>[2x]ADILPANYVVKDRWKVLKKIGGGGFGEIYEAMDLLTRENVALKVESAQQPKQVLKMEVAVLKKLQGKDHVCRFIGCGRNEKFNYVVMQLQGRNLADLRRSQPRGTFTLSTTLRLGKQILESIEAIHSVGFLHRDIKPSNFAMGRLPSTYRKCYMLDFGLARQYTNTTGDVRPPRNVAGFRGTVRYASVNAHKNREMGRHDDLWSLFYMLV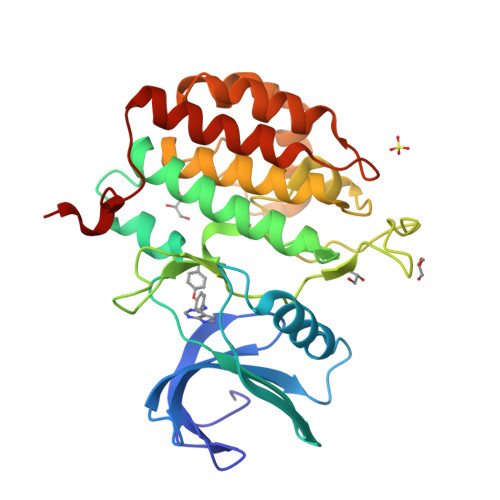EFAVGQLPWRKIKDKEQVGMIKEKYEHRMLLKHMPSEFHLFLDHIASLDYFTKPDYQLIMSVFENSMKERGIAENEAFDWEKA>[5x]QANLMRLKSDLFNRSPMYPGPTKDDPLTVTLGFTLQDIVKVDSSTNEVDLVYYEQQRWKLNSLMWDPNEYGNITDFRTSAADIW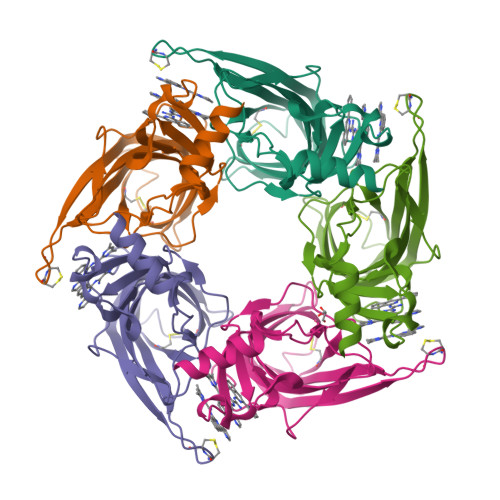TPDITAYSSTRPVQVLSPQIAVVTHDGSVMFIPAQRLSFMCDPTGVDSEEGVTCAVKFGSWVYSGFEIDLKTDTDQVDLSSYYASSKYEILSATQTRQVQHYSCCPEPYIDVNLVVKFRERRAGNGFFRNLFD>SNARDPRPLRDKNFQSAIQEEIYDYLKKNKFDIETNHPISIKFLKQPTQKGFIIIFKWLYLRLDPGYGFTKSIENEIYQILKNLRYPFLESINKSQISAVGGSNWHKFLGMLHWMVRTNIKLDMCLNKVDRSLINQNTQEITILSQPLKTLDEQDQRQERYELMVEKLLIDYFTESYKSFLKLEDNYEPSMQELKLGFEKFVHIINTDVTSTELKLEELKVDLNRKRYKLHQQVIHVIDITSKFKINIQSSLENSENELGNVIEELRNLEFE[2x];>MTSRINKPWRISHSPNSKIPSPVREKLNRLSRNQDVFPILDLQELVICLQSCDFALATQENISRPTSDYMVTLYKQIIENFMGISVESLLNSSNQETGDGHLQEENENIYLDTLNVLVLNKICFKFFENIGVQDFNMTDLYKPEAQRTQRLLSAVVNYARFREERMFDCNSFILQMESLLGQINKLNDEIKQLQKDFEVEVKEIEAAYSLLSGHINKYMNEMLEYMQ[2x];>MSQKDNLLDNPVEFLKEVRESFDIQQDVDAMKRIRHDLDVIKEESEARLKLYRSLGVILDLEND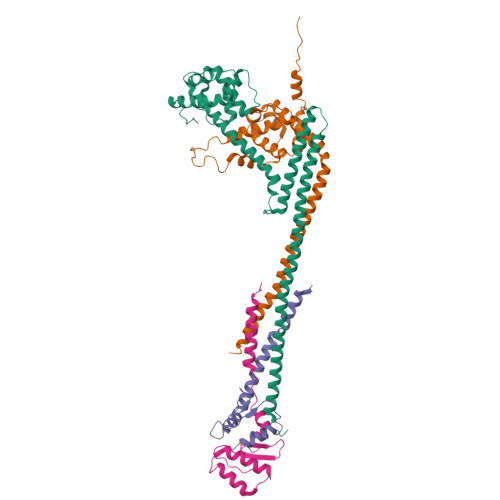QVLINRKNDGNIDILPLDNNLSDFYKTKYIWERLG[2x];>MASIDAFSDLERRMDGFQKDVAQVLARQQNHVALYERLLQLRVLPGASDVHDVRFVFGDDSRCWIEVAMHGDHVIGNSHPALDPKSRATLEHVLTVQGDLAAFLVVARDMLLAS[2x]> SNAGEIRSSVAEQEADRDIIRFGEVSFSQLAEGVWMHTTYLDLMGFGPIPSNGLLVVNGDNTILVDTAWTDEQTEQIVAWASMVLAKPVRAAVVTHAHQDKMGGMAALHGANIATWAHPLSNELAPEEGLVPARNAITFDANGWATGEA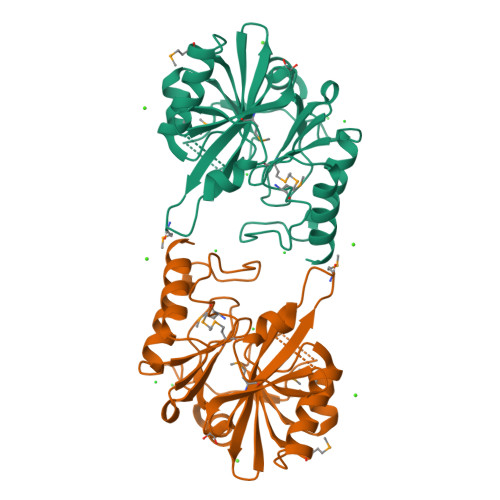AQSLAPLRLYYPGGAHTRDNITVGLPELGIAFGGCMIKAGDASNLGNLADADTAAYAQSVRNFAAAFPDARTIAMSHSPPEGRKAIERTLDLAEEL>[2x]QR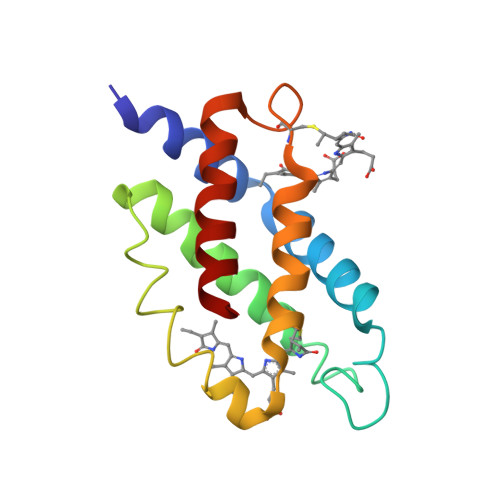AAARLEAAEKLGSNHEAVVKEAGDACFSKYGYNKNPGEAGENQEKINKCYRDIDHYMRLINYTLVVGGTGPLDEWGIAGAREVYRTLNLPSAAYIAAFVFTRDRLCAPRDMSAQAGVEFCTALDYLINSLS> SKKSGKSAKSKEKQEKITDTFKVKRKVDRFNGVSEAELLTKTLPDILTFNLDIVIIGINPGLMAAYKGHHYPGPGNHFWKCLFMSGLSEVQLNHMDDHTLPGKYGIGFTNMVERTTPGSKDLSSKEFREGGRILVQKLQKYQPRIAVFNGKCIYEIFSKEVFGVKVKNLEFGLQPHKIPDTETLCYVMPSSSARCAQFPRAQDKVHYYIKLKDLRD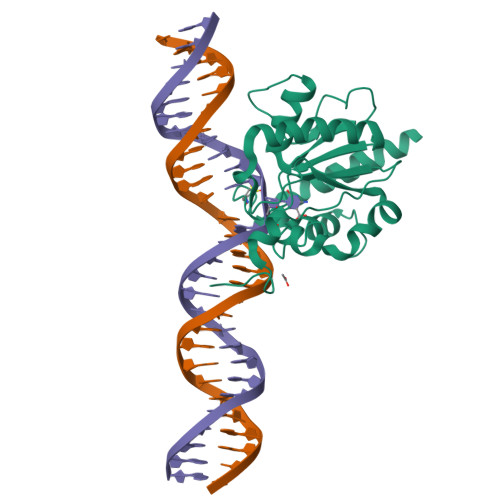QLKGIERNMDV N-{5-[(3S,4R)-1-[(3R)-3-amino-4-(4-chlorophenyl)butanoyl]-4-(hydroxymethyl)pyrrolidin-3-yl]-2-chlorophenyl}-2-(4-fluorophenyl)acetamide 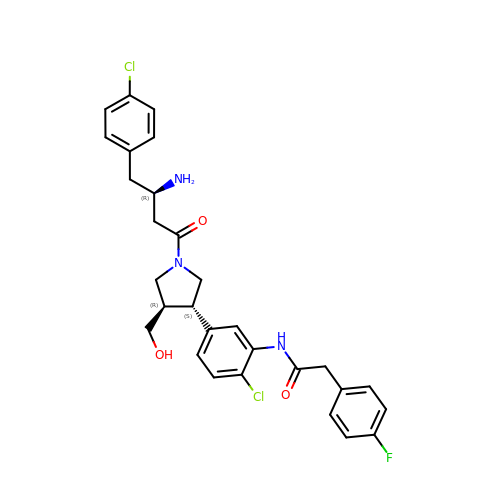| C29 H30 Cl2 F N3 O3 | UXESSWKATFQQDS-NQHRYMMQSA-N N~2~-(2,3-dichlorophenyl)-N-[2-(pyridin-4-yl)-1,3-benzoxazol-5-yl]-L-alaninamide | C21 H16 Cl2 N4 O2 | 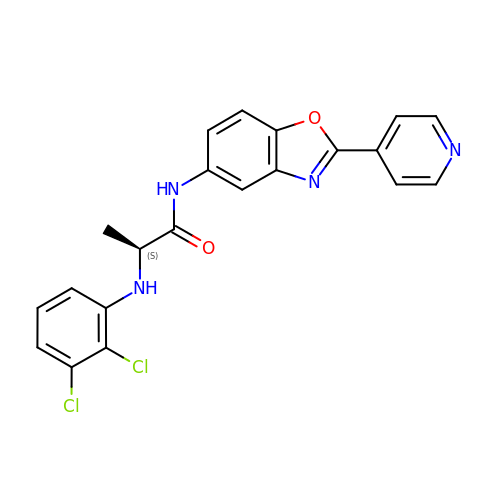IMBVKBZWLRXRAW-LBPRGKRZSA-N> MPEPTADAPTVPKARSCPFLPPDGIADIRAAAPVTRATFTSGHEAWLVTGYEEVRALLRDSSFSVQVPHALATQDGVVTQKPGRGSLLWQDEPEHTSDRKLLAKEFTVRRMQALRPNIQRIVDEHLDAIEARGGPVDLVKTFANAVPSMVISDLFGVPVERRAEFQDIAEAMMRVDQDAAATEAAGMRLGGLLYQLVQERRANPGDDLISALITTEDPDGVVDDMFLMNAAGTLLIAAHDTTACMIGLGTALLLDSPDQLALLREDPSLVGNAVEELLRYLTIGQFGGERVATRDVELGGVRIAKGEQVVAHVLAADFDPAFVEEPERFDITRRPAPHLAFGFGAHQCIGQQLARIELQIVFETLFRRLPGLRL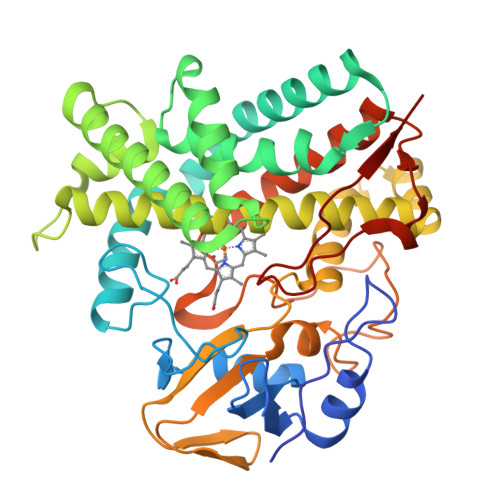AKPVEELRFRHDMVFYGVHELPVTWHHHH>[10x]GAMGMKQYIWLNETIKSNKQLAGPRGSYKRPVSVDIFRSSTILDPDKNYLLIVEEFHLHKIRLPLFKPAGHDYQVGIFNRSTDEIMGVREVDFSTFVDEDGYMYDYVDVGTAINETLAGLCDGIIGEEDIPVFSFNKHSKKFEITTTENFRNGHFIMFNDDMRVDFNSFEFDDIDEEYSLVILNEDVETQDASTLEFLTPISHIVIESNDLPVSYELLPS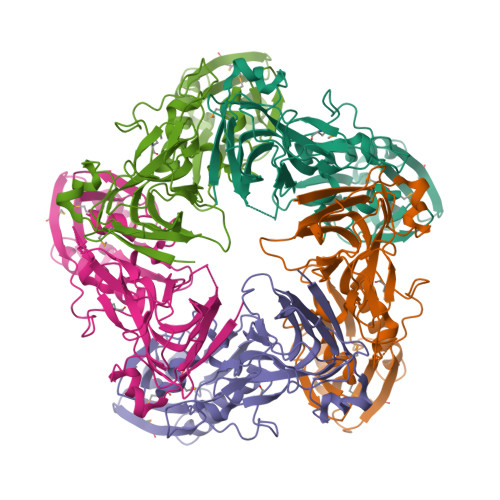ISKNTTISDNTGVFLTNYKYLQQNNQDYNSILFRVENSSNKYHNILQTNFNRFNLSFTIYDYDNEKHPLTLLPQTVIQLKLLFESID>GTTTTG[2x];>CAAAAC[2x]

A linker unit was designed and synthesized that can serve both as a hairpin turn in a DNA duplex and anchor point for an aromatic helical foldamer mimicking the shape and surface properties of B‐DNA. Here, we report how we successfully reached this milestone through the design and synthesis of a linker that can serve as both a B‐DNA duplex hairpin turn and a single helical (MQ)n extension, thereby placing the grooves and arrays of negative charges of the two segments in register. Furthermore, X possesses two hydroxy‐terminated side chains so that it can be inserted in a DNA sequence via phosphodiester linkages and serve as a hairpin turn within a unimolecular duplex. We have designed and synthesized an artificial linker based on a diamide quinoline unit that can be incorporated into DNA by standard phosphoramidite synthesis and that promotes a DNA hairpin structure.

Sequence 13, where X links complementary d(GT4G) and d(CA4C) segments was specifically prepared for structural investigations because related sequences with a stilbenediether linker had been shown to form particularly stable hairpins and to produce crystals suitable for X‐ray diffraction (XRD) analysis. The melting temperature of 13 was measured at 78 °C, while the d(GT5G)•d(CA5C) duplex is not expected to be stable at room temperature, indicating a considerable stabilization. However, single crystal XRD only showed a weak DNA fiber‐like diffraction pattern. Encouraged by our previous success in crystallizing diverse DNA sequences using racemic DNA mixtures, we prepared 14, the lll enantiomer of 13. Crystals of the 13+14 racemate diffracting to a resolution of 2.5 Å were obtained readily and the structure could be solved in centrosymmetric space group P‐1 using an earlier structure as molecular replacement model (Figures 3b‐d, S6‐S10 and Table S2). The asymmetric unit consisted of two independent molecules and four Mg2+ ions. Both molecules adopted a hairpin B‐form DNA conformation albeit with some variations of sugar puckering (Tables S3‐S7) However, the structure of the two hairpins differed significantly for both the DNA components and the X linker. Highlighting these differences, the root mean square deviation of the two hairpins superimposed based on calculations performed for all DNA atoms was 1.27 Å. Importantly, in both molecules, the quinoline rings of X linkers are coplanar and stacked to the adjacent dG−dC bp in the predicted preferred orientation. The X units have different twist angles with respect to the dG−dC bp but in both cases, this twist extends the twist between DNA bps.> ISGGDAIYSSTGRCSLGFNVRSGSTYYFLTAGHCTDGATTWWANSARTTVLGTTSGSSFPNNDYGIVRYTNTTIPKDGTVGGQDITSAANATVGMAVTRRGSTTGTHSGSVTALNATVNYGGGDVVYGMIRTNVCAEPGDSGGPLYSGTRAIGLTSGGSGNCSSGGTTFFQPVTEALVAYGVSVY;> VDCSEYPKPAC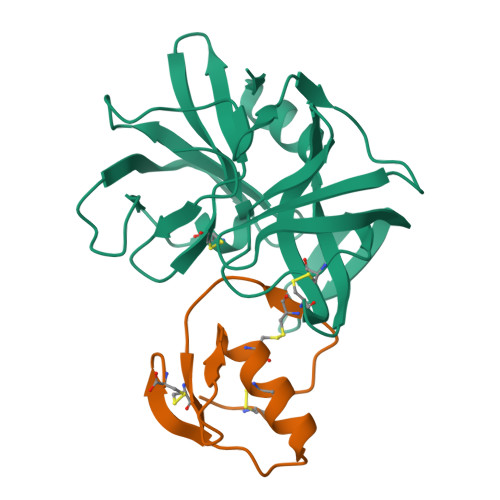TSEYRPLCGSDNKTYGNKCNFCNAVVESNGTLTLSHFGKC>[6x]MRLKKLYLKGFKSFGRPSLIGFSDRVTAIVGPNGSGKSNIIDAIKWVFGEQSKKELRASEKFDMIFAGSENLPPAGSAYVELVFEENGEEITVARELKRTGENTYYLNGSPVRLKDIRDRFAGTGLGVDFYSIVGQGQIDRIVNASPEELRLESSKHP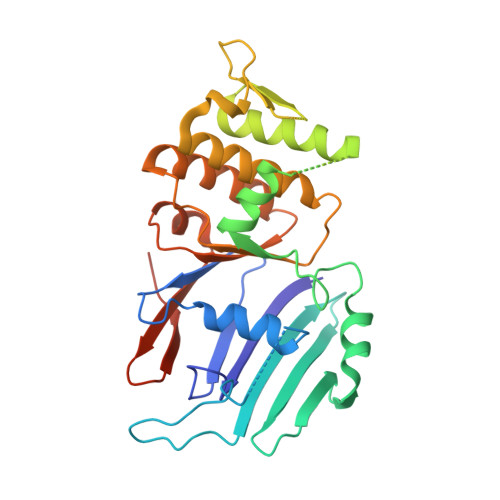TSLVPRGSYQRVNESFNRFISLLFFGGEGRLNIVSEAKSILDAGFEISIRKPGRRDQKLSLLSGGEKALVGLALLFALMEIKPSPFYVLDEVDSPLDDYNAERFKRLLKENSKHTQFIVITHNKIVMEAADLLHGVTMVNGVSAIVPVEVEKILEVGSHHHHHH>M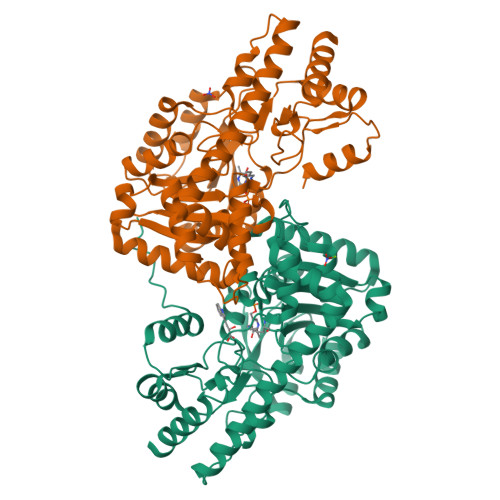FERIDYYAGDPILGLVEKFAADNNPDKVNLGIGIYYDESGVMPVLDCVKIAEQRIADPISPRPYLPMAGLPGHRKGCQELLFGKDAPVLKDGLVATIATIGGSGALKVGAEFIHEWFPQSKCYVSDPTWGNHIAIFEGCDIEVGKYPYYDTATGGIKFDEMIAFFETLNKDDVLLLHPCCHNPTGVDLTREQWDTVLNVIQERELIPFMDIAYQGFGEDMDSDAYAIRKAVDMGLPLFVSNSFSKNLSLYGERVGGLSVVCPTVDETERVFGQLNSTVRRIYSSPPSHGGRVVDIVMNDAALHEQWVGEVYAMRDRIKSMRTKLKSVLEAKISGRNFDYLTAQNGMFSFTGLTPEQVERLQSEFGIYMISNSRMCVAGLNSSNIDYVANAMVDVLKD[4x]>[3x]MGSDKIHHHHHHMKIDLIISADDIKEEKVKNKTAVVIDMLRATSVITTALNNGCKRVVPVLTVEEALKKVKEYGKDAILGGERKGLKIEGFDFSNSPMEY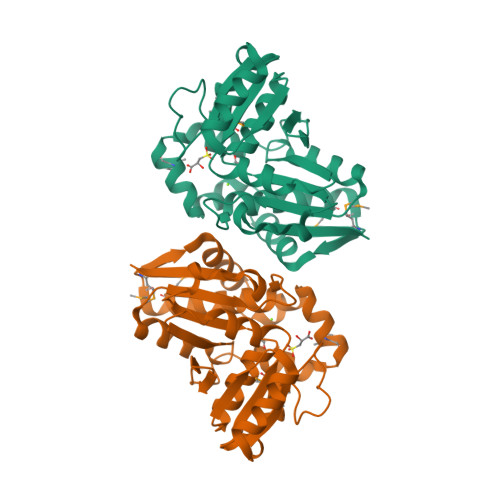TEDVVKGKTLIMTTTNGTRAIKGSETARDILIGSVLNGEAVAEKIVELNNDVVIVNAGTYGEFSIDDFICSGYIINCVMDRMKKLELTDAATTAQYVYKTNEDIKGFVKYAKHYKRIMELGLKKDFEYCCKKDIVKLVPQYTNGEIL> GPLGSETITVPTPIKQIFSDDAFAETIKDNLKKKSVTDAVTQNELNSIDQIIANNSDIKSVQGIQYLPNVTKLFLNGNKLTDIKPLANLKNLGWLFLDENKVKDLSSLKDLKKLKSLSLEHNGISDINGLVHLPQLE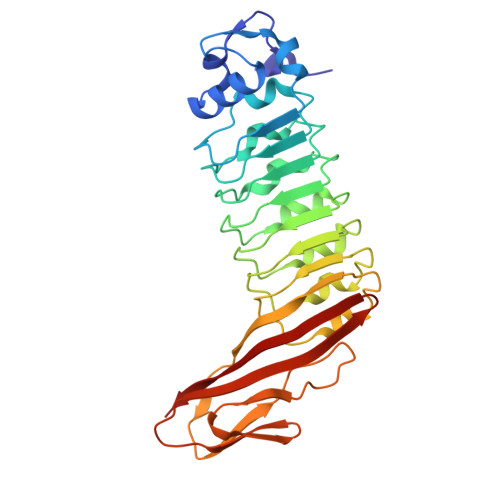SLYLGNNKITDITVLSRLTKLDTLSLEDNQISDIVPLAGLTKLQNLYLSKNHISDLRALAGLKNLDVLELFSQECLNKPINHQSNLVVPNTVKNTDGSLVTPEIISDDGDYEKPNVKWHLPEFTNEVSFIFYQPVTIGKAKARFHGRVTQPLKE> MFNKSVNSGFTFGNQNTSTPTSTPAQPSSSLQFPQKSTGLFGNVNVNANTSTPSPSGGLFNANSNANSISQQPANNSLFGNKPAQPSGGLFGATNNTTSKSAGSLFGNNNATANSTGSTGLFSGSNNIASSTQNGGLFGNSNNNNITSTTQNGGLFGKPTTTPAGAGGLFGNSSSTNSTTGLFGSNNTQSSTGIFGQKPGASTTGGLFGNNGASFPRSGETTGTMSTNPYGINISNVPMAVADMPRSITSSLSDVNGKSDAEPKPIENRRTYSFSSSVSGNAPLPLASQSSLVSRLSTRLKATQKSTSPNEIFSPSYSKPWLNGAGSAPLVDDFFSSKMTSLAPNENSIFPQNGFNFLSSQRADLTELRKLKIDSNRSAAKKLKLLSGTPAITKKHMQDEQDSSENEPIANADSVTNIDRKENRDNNLDNTYLNGKEQSNNLNKQDGENTLQHEKSSSFGYWCSPSPEQLERLSLKQLAAVSNFVIGRRGYGCITFQHDVDLTAFTKSFREELFGKIVIFRSSKTVEVYPDEATKPMIGHGLNVPAIITLENVYPVDKKTKKPMKDTTKFAEFQVFDRKLRSMREMNYISYNPFGGTWTFKVNHFSIWGLVNEEDAEIDEDDLSKQEDGGEQPLRKVRTLAQSKPSDKEVILKTDGTFGTLSGKDDSIVEEKAYEPDLSDADFEGIEASPKLDVSKDWVEQLILAGSSLRSVFATSKEFDGPCQNEIDLLFSECNDEIDNAKLIMKERRFTASYTFAKFSTGSMLLTKDIVGKSGVSIKRLPTELQRKFLFDDVYLDKEIEKVTIEARKSNPYPQISESSLLFKDALDYMEKTSSDYNLWKLSSILFDPVSYPYKTDNDQVKMALLKKERHCRLTSWIVSQIGPEIEEKIRNSSNEIEQIFLYLLLNDVVRASKLAIESKNGHLSVLISYLGSNDPRIRDLAELQLQKWSTGGCSIDKNISKIYKLLSGSPFEGLFSLKELESEFSWLCLLNLTLCYGQIDEYSLESLVQSHLDKFSLPYDDPIGVIFQLYAANENTEKLYKEVRQRTNALDVQFCWYLIQTLRFNGTRVFSKETSDEATFAFAAQLEFAQLHGHSLFVSCFLNDDKAAEDTIKRLVMREITLLRASTNDHILNRLKIPSQLIFNAQALK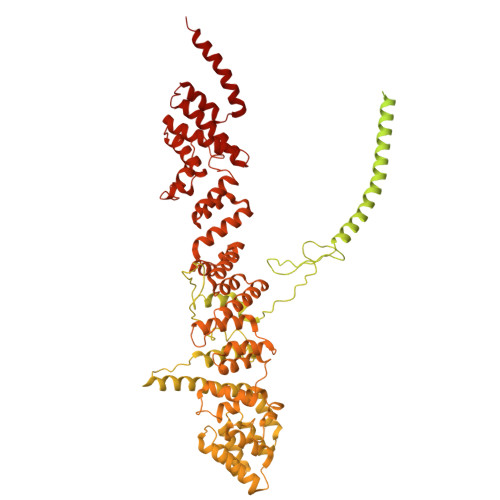DRYEGNYLSEVQNLLLGSSYDLAEMAIVTSLGPRLLLSNNPVQNNELKTLREILNEFPDSERDKWSVSINVFEVYLKLVLDNVETQETIDSLISGMKIFYDQYKHCREVAACCNVMSQEIVSKILEKNNPSIGDSKAKLLELPLGQPEKAYLRGEFAQDLMKCTYKI> TARYGVSNT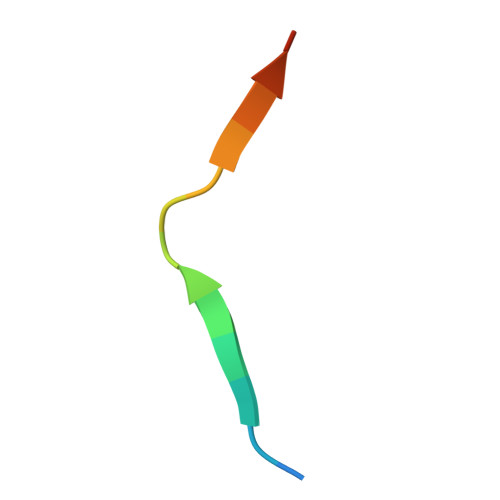SINRKKP> GIDPFTKSELAVEILEKGQVRFWMQAEKLSGNAKVNYIFNEKEIFEGPKYKMHIDRNTGIIEMFMEKLQDEDEGTYTFQLQDGKATNHSTVVLVGDVFKKLQKEAEFQRQEWIRKQGPHFVEYLSWEVTGECNVLLKCKVANIKKETHIVWYKDEREISVDEKHDFKDGICTLLITEFSKKDAGIYEVILKDDRGKDKSRLKLVDEA

Members of the myomesin protein family function as molecular bridges that connect major filament systems in the central M-band of muscle sarcomeres, which is a central locus of passive stress sensing. To unravel the mechanism of molecular elasticity in such filament-connecting proteins, we have determined the overall architecture of the complete C-terminal immunoglobulin domain array of myomesin by X-ray crystallography, electron microscopy, solution X-ray scattering, and atomic force microscopy. Our data reveal a dimeric tail-to-tail filament structure of about 360 Å in length, which is folded into an irregular superhelical coil arrangement of almost identical α-helix/domain modules. The myomesin filament can be stretched to about 2.5-fold its original length by reversible unfolding of these linkers, a mechanism that to our knowledge has not been observed previously.

First, we determined the overall architecture of the complete myomesin domain array, including Ig domains My9–My10–My11–My12–My13, from crystal structures of a total of three filament fragments: the My9–My11 triplet, determined at 2.5 Å resolution; the My10–My11 doublet, at 1.9 Å resolution; and the homodimeric My11–My13 triplet at 3.5 Å resolution. Remarkably, all five Ig domains of the myomesin filament are connected by α-helices that are identical in terms of orientation with respect to the preceding Ig domain, and they form a substantial, structurally highly conserved Ig domain/helix interface with an area of 350–600 Å2. By contrast, we have observed neither a common interface nor a similar orientation for any of the My–My domain-connecting helices and subsequent Ig domains My10, My11, My12, and My13. As the overall geometry of the IgH segments is rigid, the limited variability in terms of arrangements of neighboring My domains originates from the diverse helix/My domain connections. Whereas long six-turn helices are found in the My10–My11 and My12–My13 connecting segments, the corresponding helices in the other two connecting segments, My9–My10 and My11–My12, are slightly shorter, with about four turns each. Because of the smaller length of their linkers, My9–My10 and My11–My12 show limited direct interactions in their respective Ig doublets, whereas in the other two doublets, My10–My11 and My12–My13, the neighboring My domains are too far away from each other to form an interface.> SGNLESSLAPISAKDMLDYLACKDKKPTDVVKSHTEVENGKIVRVKCGDIVALVQKAREQSGDAWQ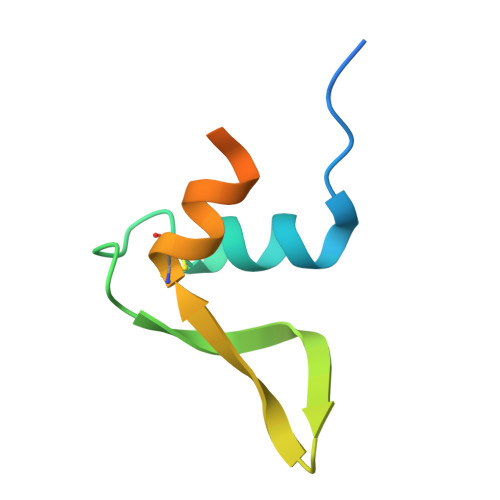GGY> MNQIWLKVCAASDMQPGTIRRVNRVGAAPLAVYRVGDQFYATEDTCTHGIAS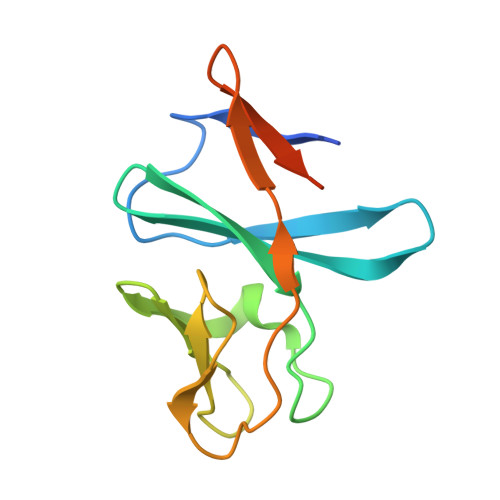LSEGTLDGDVIECPFHGGAFNVCTGMPASSPCTVPLGVFEVEVKEGEVYVAGEKKLEHHHHHH>MSYQSTIVPVELHSFEDAQVIGGAFRDGDAVVFDMSLLSREEARRIVDFAAGLCFALRGKMQKIDSVTFAVVPELSNISTSELERAARIR[2x]

At the cell division site, FtsZ protofilaments form a highly dynamic, membrane-bound structure, the Z-ring, which serves as a scaffold for the recruitment of the extra-cytoplasmic cell wall biosynthetic machinery. Here we investigate the physiological function of Corynebacterium glutamicum SepF, the only cell division-associated protein from Actinobacteria known to interact with the conserved C-terminal tail of FtsZ. Our structural data revealed the FtsZ-binding pocket, defining the SepF homodimer as the functional unit, and suggesting a reversible β-sheet-mediated oligomerization interface possibly regulated via an alpha helical switch. We found that FtsZ filaments and lipid membranes have opposing effects on SepF polymerization, pointing to a complex dynamic role of the protein at the division site, involving FtsZ bundling, Z-ring tethering and membrane reshaping activities that are needed for proper Z-ring assembly and function.

Helix α3 formation and stabilization were not due to FtsZ binding, because the crystal structure of unliganded SepFΔML revealed the same overall structure than FtsZCTD-bound SepFΔML (rmsd of 0.83 Å for 160 equivalent Cα atoms in the homodimer), indicating that peptide binding produced no significant conformational changes. The presence of this helix has important functional implications as it caps the β-sheet that was previously described as the dimerization interface of B. subtilis SepF11. If the functional SepF unit is conserved, the β-sheet-mediated interface observed in B. subtilis SepF crystals could therefore mediate protein polymerization in solution. This interface, which was also seen in SepF-like proteins from Pyrococcus furiosus and Archaeoglobus fulgidus, is precluded in the C. glutamicum SepF structure by the presence of the C-terminal helix α3. However, inspection of the unliganded SepFΔML structure revealed that this helix displays considerably higher B-factor values than the rest of the protein and a similar trend is also observed in the SepFΔML–FtsZCTD complex, suggesting that helix α3 could play a regulatory role on SepF polymerization by uncovering the outer face of the β-sheet for intermolecular interactions.The OXA-48 carbapenemase is widely disseminated in Enterobacterales, necessitating new treatments for producer strains. OXA-48 is a class D SBL that uses a nucleophilic serine (Ser70) to hydrolyse β-lactams, with a proximal post-translationally carbamylated lysine (Lys73) proposed to act as the general base for both the acylation and deacylation steps of the reaction. Diazabicyclooctane (DBO) inhibitors, including avibactam and nacubactam, act on a wide range of enzymes to overcome β-lactamase-mediated resistance. Here we describe investigations on how avibactam and nacubactam inhibit OXA-48 and two variants, OXA-163 and OXA-405, with deletions in the β5–β6 loop neighbouring the active site that modify activity towards different β-lactam classes.

Nacubactam is distinguished from avibactam by an extended C2 substituent bearing a 1-aminoethoxy group. Both OXA-163 and OXA-405 have four amino acid deletions within the β5–β6 loop, including of residue Arg214. Crystal structures were obtained for OXA-163 and OXA-405, as uncomplexed enzymes and in the nacubactam- and avibactam-bound forms. Both OXA-163 and OXA-405 assemble as homodimers in the asymmetric unit. Consistent with their high overall sequence identities, they adopt very similar overall folds and active site arrangements compared to OXA-48. The exception is the Ser70 nucleophile, which is in dual conformations in one of the two chains in the crystallographic dimers of uncomplexed OXA-163 and OXA-405. The respective protein backbones only differ at the β5–β6 loop, which is truncated in the cases of OXA-163 and OXA-405, compared to OXA-48. Part of the OXA-405 β7–α10 loop, which neighbours the β5–β6 loop, could not be modelled due to weak electron density, indicating that this loop is more mobile in uncomplexed OXA-405, compared to the other enzymes. β7–α10 loop flexibility coincides with the presence of an alternative side chain rotamer for Tyr211 in the OXA-405:nacubactam complex.

>[2x]GPKEWQENKSWNAHFTEHKSQGVVVLWNENKQQGFTNNLKRANQAFLPASTFKIPNSLIALDLGVVKDEHQVFKWDGQTRDIATWNRDHNLITAMKYSVVPVYQEFARQIGEARMSKMLHAFDYGNEDISGNVDSFWLDGGIRISATEQISFLRKLYHNKLHVSERSQRIVKQAMLTEANGDYIIRAKTGYSPKIGWWVGWVELDDNVWFFAMNMDMPTSDGLGLRQAITKEVLKQEKIIP> ADGRSTRYWNCCKPSCGWAKKAP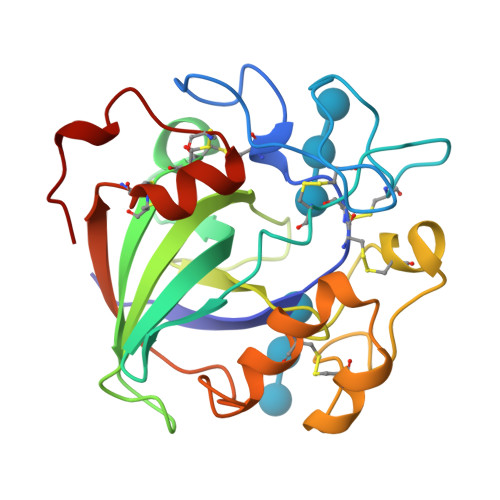VNQPVFSCNANFQRITDFDAKSGCEPGGVAYSCADQTPWAVNDDFALGFAATSIAGSNEAGWCCACYELTFTSGPVAGKKMVVQSTSTGGDLGSNHFDLNIPGGGVGIFDGCTPQFGGLPGQRYGGISSRNECDRFPDALKPGCYWRFDWFKNADNPSFSFRQVQCPAELVARTGCRRNDDGNFPAV> MAQLTHINAAGEAHMVDVSAKAETVREARAEAFVTMRSETLAMIIDGRHHKGDVFATARIAGIQAAKRTWDLIPLCHPLMLSKVEVNLQAEPEHNRVRIETLCRLTGKTGVEMEALTAASVAALTIYAMCKAVQ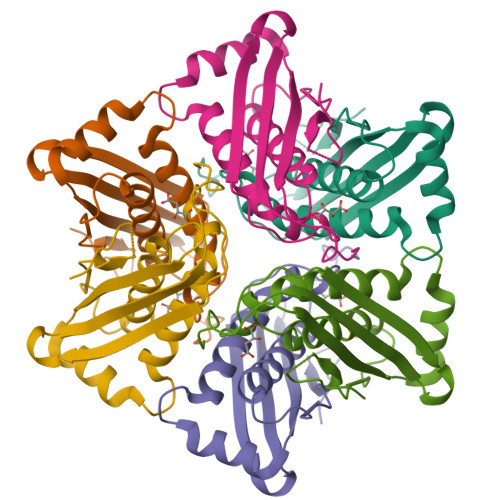KDMVIGPVRLLAKSGGKSGDFKVEADD>[2x]MASSYSASAEPARVRALVYGHHGDPAKVVELKNLELAAVRGSDVRVKMLAAPINPSDINMIQGNYGLLPELPAVGGNEGVAQVVAVGSNVTGLKPGDWVIPANAGLGTWRTEAVFSEEALIQVPSDIPLQSAATLGVNPCTAYRMLMDFEQLQPGDSVIQNASNS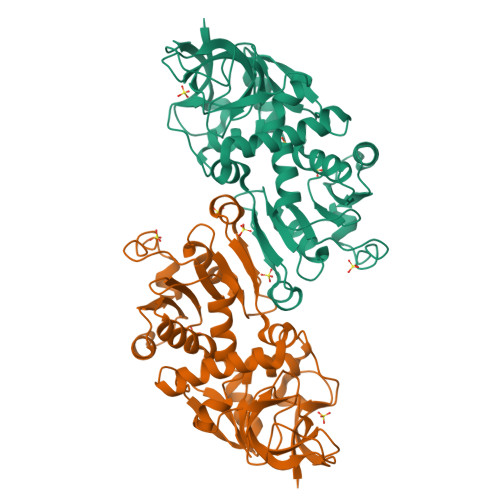GVGQAVIQIAAALGLRTINVVRDRPDIQKLSDRLKSLGAEHVITEEELRRPEMKNFFKDMPQPRLALNCVGGKSSTELLRQLARGGTMVTYGGMAKQPVVASVSLLIFKDLKLRGFWLSQWKKDHSPDQFKELILTLCDLIRRGQLTAPACSQVPLQDYQSALEASMKPFISSKQILTM> MAETSEEVAVLVQRVVKDITNAFRRNPHIDEIGLIPCPEARYNRSPIVLVENKLGVESWCVKFLLPYVHNKLLLYRTRKQWLNRDELIDVTCTLLLLNPDFTTAWNVRKELILSGTLNPIKDLHLGKLALTKFPKSPETWIHRRWVLQQLIQETSLPSFVTKGNLGT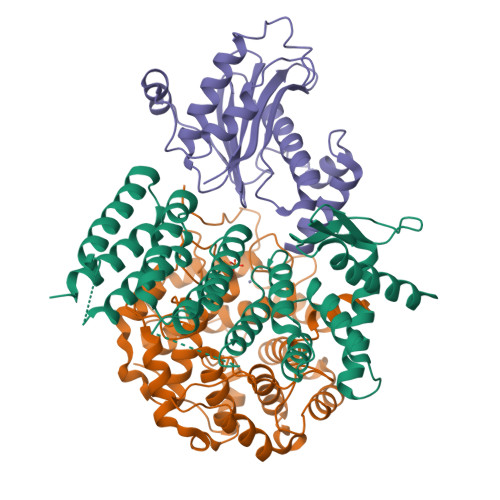IPTERAQRLIQEEMEVCGEAAGRYPSNYNAWSHRIWVLQHLAKLDVKILLDELSSTKHWASMHVSDHSGFHYRQFLLKSLISQTVIDSSVMEQNPLRSEPALVPPKDEEAAVSTEEPRINLPHLLEEEVEFSTDLIDSYPGHETLWCHRRHIFYLQHHLN;> GPLGSMGTPQKDVIIKSDAPDTLLLEKHADYIASYGSKKDDYEYCMSEYLRMSGIYWGLTVMDLMGQLHRMNREEILAFIKSCQHECGGISASIGHDPHLLYTLSAVQILTLYDSINVIDVNKVVEYVKGLQKEDGSFAGDIWGEIDTRFSFCAVATLALLGKLDAINVEKAIEFVLSCMNFDGGFGCRPGSESHAGQIYCCTGFLAITSQLHQVNSDLLGWWLCERQLPSGGLNGRPEKLPDVCYSWWVLASLKIIGRLHWIDREKLRNFILACQDEETGGFADRPGDMVDPFHTLFGIAGLSLLGEEQIKPVNPVFCMPEEVLQRVNVQPELVS;> MKLYSLSVLYKGEAKVVLLKAAYDVSSFSFFQRSSVQEFMTFTSQLIVERSSKGTRASVKEQDYLCHVYVRNDSLAGVVIADNEYPSRVAFTLLEKVLDEFSKQVDRIDWPVGSPATIHYPALDGHLSRYQNPREADPMTKVQAELDETKIILHNTMESLLERGEKLDDLVSKSEVLGTQSKAFYKTARKQNSCCAIM> MLTEEFVSAICGPPLSSNTAIAKDVGIYCHTLSPSYSVKSTFKKSSVPVNCLAVSDTHIFAGQHEKAYVHVYSRLRGNQEAFVALPERIRCLILIGDILVVGTTEGRLMLWEICTGRLVSTPARHVQAVSCVAATPSHVLTGSDDSDIHVWSLSQLLELDSAAEHEPLRTLANHRAAITALAVSPSDSADTNFCVSASKDKSCIIWNYQTGDALRTL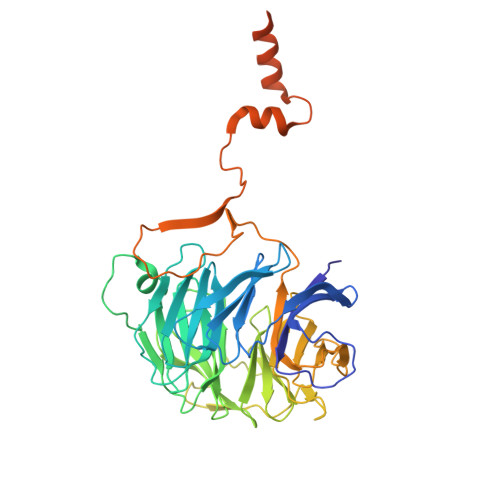IFPGYPLCMSLDPSSRAIFVSCEDSSLYVAEMFGEKPLLGPGSEDPSTVVQISTPFGATQPDVGPASCLSVSYDGTMLLTGHPRGQIMRWDISENKSPVELANLNAAVTNLIFVSPFLTSKPTKTVNIIKPSQAERAYTFTAQFEPMSFTKSRLDSLLNATGFPADALESAIVAFYQPVTQSAGDQELQRQNEELWEIINEQRALQKETLQRYVEAKSSR>[4x]MGQGDESERIVINVGGTRHQTYRSTLRTLPGTRLAWLAEPDAHSHFDYDPRADEFFFDRHPGVFAHILNYYRTGKLHCPADVCGPLYEEELAFWGIDETDVEPCCWMTYRQHRDAEEALDSFGGAPLDNSADDADADGPGDSGDGEDELEMTKRLALSDSPDGRPGGFWRRWQPRIWALFEDPYSSRYARYVAFASLFFILVSITTFCLETHERFNPIVNKTEIENVRNGTQVRYYREAETEAFLTYIEGVCVVWFTFEFLMRVIFCPNKVEFIKNSLNIIDFVAILPFYLEVGLSGLSSKAAKDVLGFLRVVRFVRILRIFKLTRHFVGLRVLGHTLRASTNEFLLLIIFLALGVLIFATMIYYAERIGAQP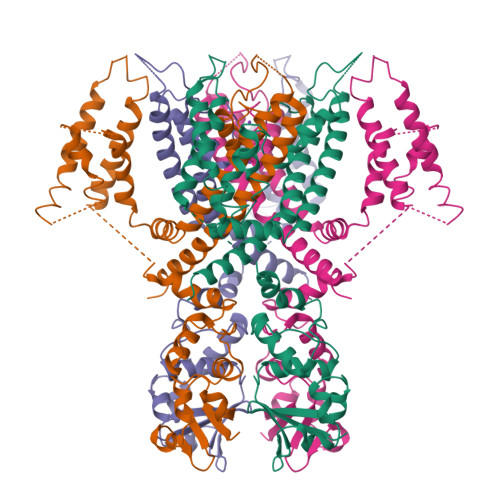NDPSASEHTHFKNIPIGFWWAVVTMTTLGYGDMYPQTWSGMLVGALCALAGVLTIAMPVPVIVNNFGMYYSLAMAKQKLPKKKKKHIPRPPQLGSPNYCKSVVNSPHHSTQSDTCPLAQEEILEINRAGRKPLRGMSIGSLEVLFQ>MGSSHHHHHHSSGENLYFQGSEELQNKLEDVVIDRNLLILGKILGEGEFGSVMEGNLKQEDGTSLKVAVKTMKLDNSSQREIEEFLSEAACMKDFSHPNVMRLLGVCIEMSSQGIPKPMVILPFMKYGDLHTYLLYSRLETGPKHIPLQTLLKFMVDIALGMEYLSNRNFLHRDLAARNCMLRDDMTVCVADFGLSKKIYSGDYYRQGRIAKMPVKWIAIESLADRVYTSKSDVWAFGVTMWEIATRGMTPYPGVQNHEMYDYL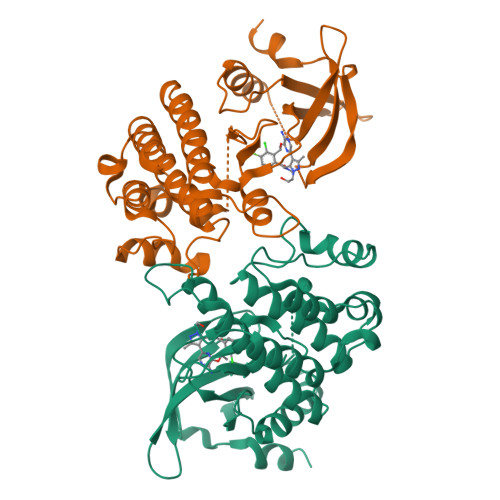LHGHRLKQPEDCLDELYEIMYSCWRTDPLDRPTFSVLRLQLEKLLESLPDV[2x]> GMSHVSYAEPPAQGWDIHCHTVFSDGTETPRTLVEQARKLGLHGVAIADHDTTAGWDEATEASEEIGLPLLLGTEITAVDEDVSVHMLAFQYDPSNEHISSMFANTRAARLRRTKRMVERLSQDFPITWDDVLAQVKEGERTTIGRPHIADALVAAGVYETRSDAFADAVSAKSKYYIPTPSPSTHEVIAAVKGAGGVV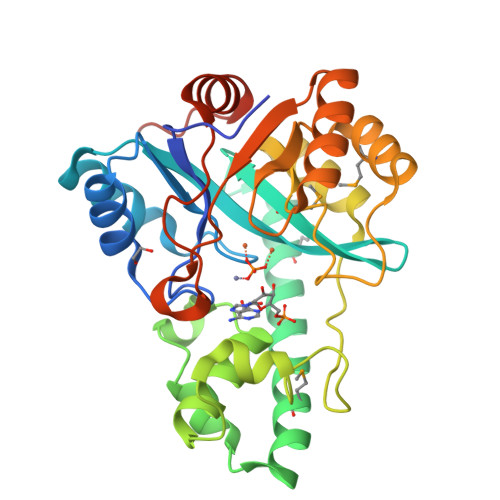VAAHAGDPQRNRRLLSDEQLDAMIADGLDGLEVWHRGNPPEQRERLLTIAARHDLLVTGGSDWHGKGKPNGLGENLTDDDTVREILCRGVDLIGRVGSSHAA> GPLGSKEISEADKVIKATKETKETKKEVKRLKKEAKQRQQIPDHKKPQYASVDDTKTQALFDIYDTLNVNDKSFGDWFGNSALKDKTYLYAMDLLDYNNYLSIENPIIKTRAMGTYADLIIITGSLEQVNGYYNILKALNKRNAKFVLKINENMPYAQA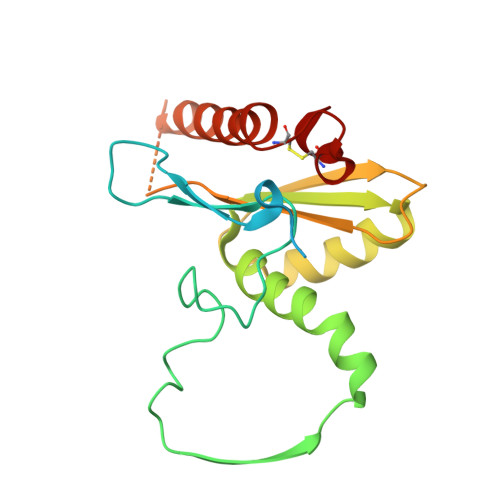TFLRVPKRSDPNAHTLDKGASIDENKLFEQQKRAYFNYANDVICRPNDEVCSPLRD> SMSTNGDDHQVKDSLEQLRCHFTWELSIDDDEMPDLENRVLDQIEFLDTKYSVGIHNLLAYVKHLKGQNEEALKSLKEAENLMQEEHDNQANVRSLVTWGNFAWMYYHMGRLAEAQTYLDKVENICKKLSNPFRYRMECPEIDCEEGWALLKCGGKNYERAKACFEKVLEVDPENPESSAGYAISAYRLDGFKLATKNHKPFSLLPLRQAVRLNPDAGYIKVLLALKLQDEGQEAEGEKYIEEALANMSSQTYVFRYAAKFYRRKGSVDKALELLKKALQETPTSVLLHHQIGLCYKAQMIQIKEATKGQPRGQNREKLDKMI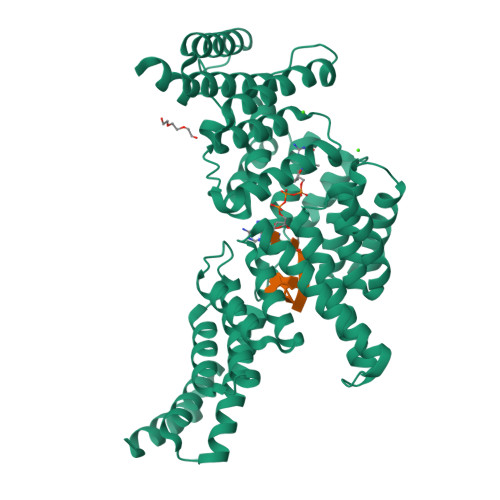RSAIFHFESAVEKKPTFEVAHLDLARMYIEAGNHRKAEENFQKLLCMKPVVEETMQDIHFHYGRFQEFQKKSDVNAIIHYLKAIKIEQASLTRDKSINSLKKLVLRKLRRKALDLESLSLLGFVYKLEGNMNEAEEYYERAERLAADFENSVRQGP>[6x]MFRIGQGFDVHQ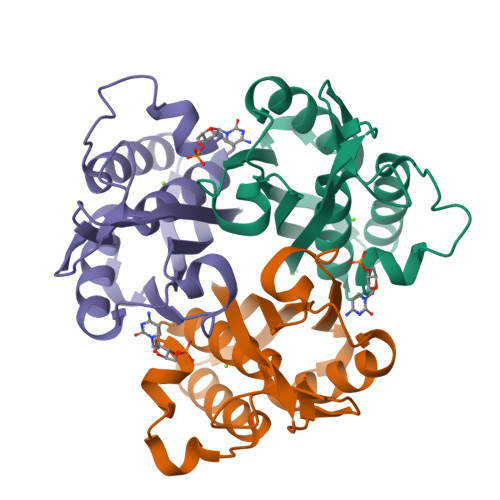LVEGRPLIIGGIEIPYEKGLLGHSDADVLLHTVADACLGAVGEGDIGKHFPDTDPEFKDADSFKLLQHVWGIVKQKGYVLGNIDCTIIAQKPKMLPYIEDMRKRIAEGLEADVSQVNVKATTTEKLGFTGRAEGIAAQATVLIQKG>GSFKEGERVLAYHGPLLYEAKVQKSENKEDEWRYHVHYLGWSKSWDEWVTNDRLLK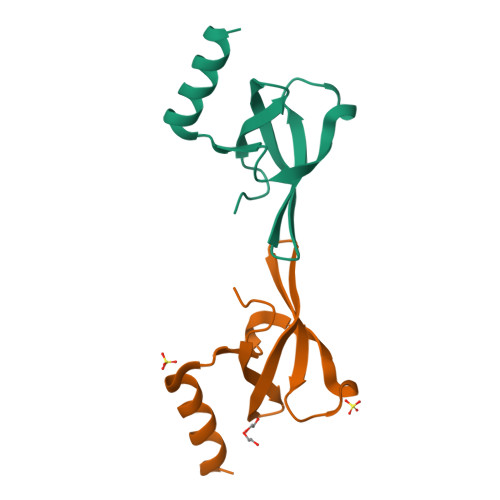LTDENIRKQQELEKSQ[2x]> QDITLYSGRGETLVKPIIEQFEKQSGIKVNVRYGDTAQLAVLLQEEGARSPADVYWGQDAGAMGALANAGLLATLPEAVYKQLPEIYTSKTGQWVAASGRSRVIAYSTERASAEDIPASVFDLTSEKYQGRFGLAPTNGGFQSFVTAMRVQHGDEKTLAWLKAMKANQPKIYRNNTTQIQAIGDGEIDFALVNNYYLPRFVAANASFPAKQTYFAEGDIGNLVNVAGVAVLKSSK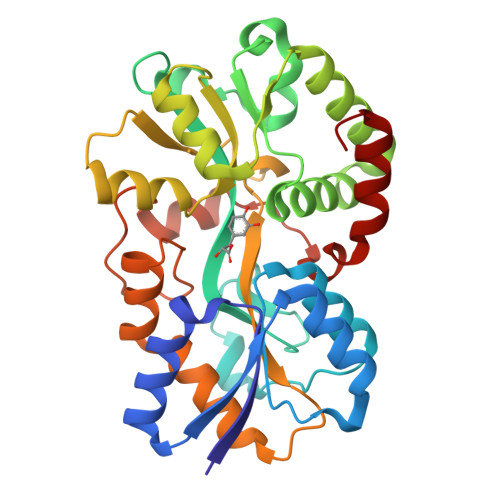KQPQAIQFIEYMLSPAAQQYFTSVVGEYPVTQGIIPNPVLGELDTLLQAAPSIDLDQLADLQGTLKLLRDAGLL> RVDVSLPGASLFSGGLHPITLMERELVEIFRALGYQAVEGPEVESEFFNFDALNIPEHHPARDMWDTFWLTGEGFRLEGPLGEEVEGRLLLRTHTSPMQVRYMVAHTPPFRIVVPGRVFRFEQTDATHEAVFHQLEGLVVGEGIAMAHLKGAIYELAQALFGPDSKVRFQPVYFPFVEPGAQFAVWWPEGGKWLELGGAGMVHPKVFQAVDAYRERLGLPPAYRGVTGFAFGLGVERLAMLRYGIPDIRYFFGGRLKFLEQFKGVL;> MRVPFSWLKAYVPELESPEVLEERLAGLGFETDRIERVFPIPRGVVFARVLEAHPIPGTRLKRLVLDAGRTVEVVSGAENARKGIGVALALPGTELPGLGQKVGERVIQGVRSFGMALSPRELGVGEYGGGLLEFPEDALPPGTPLSEAWPEEVVLDLEVTPNRPDALGLLGLARDLHALGYALVEPEAALKAEALPLPFALKVEDPEGAPHFTLGYAFGLRVAPSPLWMQRALFAAGMRPINNVVDVTNYVMLERAQPMHAFDLRFVGEGIAVRRAREGERLKTLDGVERTLHPEDLVIAGWRGEESFPLGLAGVMGGAESEVREDTEAIALEVACFDPVSIRKTARRHGLRTEASHRFERGVDPLGQVPAQRRALSLLQALAGARVAEALLEAGSPKPPEAIPFRPEYANRLLGTSYPEAEQIAILKRLGCRVEGEGPTYRVTPPSHRLDLRLEEDLVEEVARIQGYETIPLALPAFFPAPDNRGVEAPYRKEQRLREVLSGLGFQEVYTYSFMDPEDARRFRLDPPRLLLLNPLAPEKAALRTHLFPGLVRVLKENLDLDRPERALLFEVGRVFREREETHLAGLLFGEGVGLPWAKERLSGYFLLKGYLEALFARLGLAF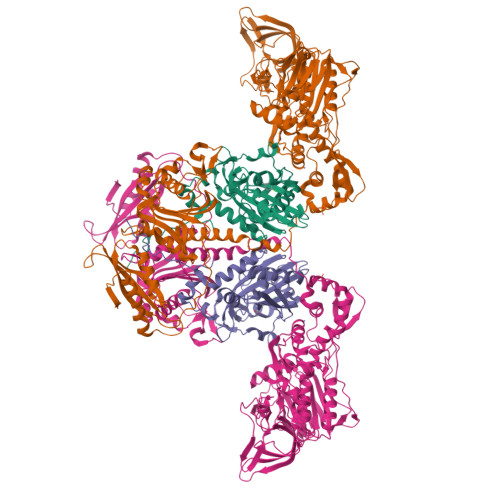RVEAQAFPFLHPGVSGRVLVEGEEVGFLGALHPEIAQELELPPVHLFELRLPLPDKPLAFQDPSRHPAAFRDLAVVVPAPTPYGEVEALVREAAGPYLESLALFDLYQGPPLPEGHKSLAFHLRFRHPKRTLRDEEVEEAVSRVAEALRARGFGLRGLDTP> GSMTAEEDMEDDTSWRSEATFQFTVERFSRLSESVLSPPCFVRNLPWKIMVMPRFYPDRPHQKSVGFFLQCNAESDSTSWSCHA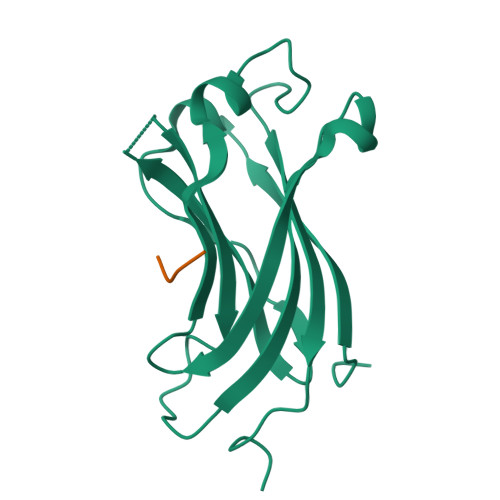QAVLKIINYRDDEKSFSRRISHLFFHKENDWGFSNFMAWSEVTDPEKGFIDDDKVTFEVFVQADAPHGVAWASTS;> DSRASTSSSS>TTNKPIVLSTWNFGLHANVEAWKVLSKGGKALDAVEKGVRLVEDDPTERSVGYGGRPDRDGRVTLDACIMDENYNIGSVACMEHIKNPISVARAVMEKTPHVMLVGDGALEFALSQGFKKENLLTAESEKEWKEWLKTSQYKPIVNIENHD[2x];>[2x]TIGMIALDAQGNLSGACTTSGMAYKMHGRVGDSPIIGAGLFVDNEIGAATATGHGEEVIRTVGTHLVVELMNQGRTPQQACKEAVERIVKIVNR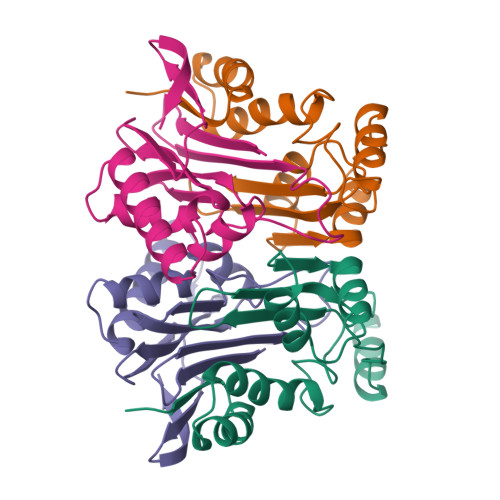RGKNLKDIQVGFIALNKKGEYGAYCIQDGFNFAVHDQKGNRLETPGFALK>[4x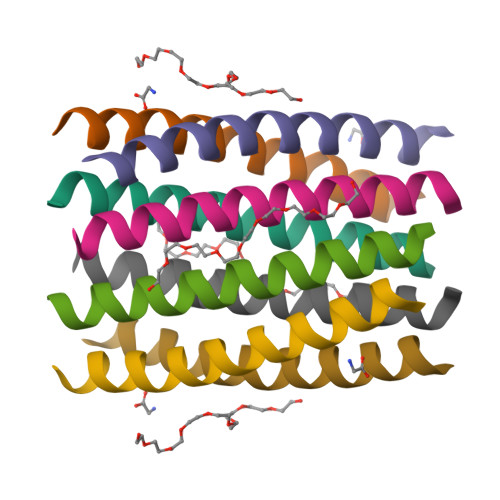]XGKKSAWATVISALATVISALATVISAWATVGX> MRSYDMNVETAAELSAVNDILASIGEPPVSTLEGDANADAANARRILNKINRQIQSRGWTFNIEEGITLLPDVYSNL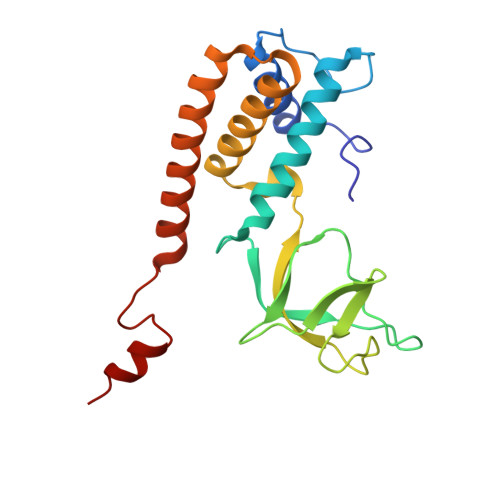IVYSDDYLSLMSTSGQSIYVNRGGYVYDRTSQSDRFDSGITVNIIRLRDYDEMPECFRYWIVTKASRQFNNRFFGAPEVEGVLQEEEDEARRLCMEYEMDYGGYNMLDGDAFTSGLLTR>[2x]MAPLENNYNESLNKSKDAIDDKTWSKLFPSIVSDPDRSSNFMIRAIYVVFSAVLRQRNILEKEYFSKNYITE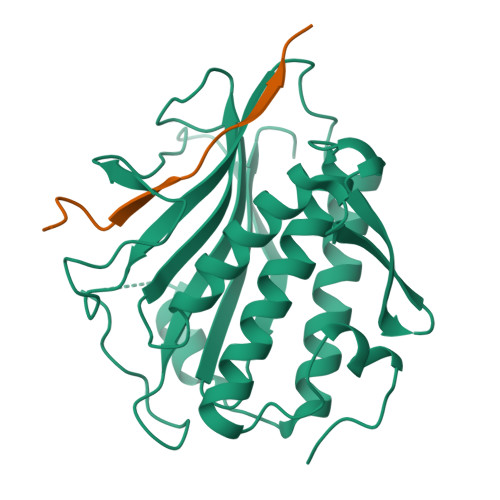NLSCMTLSFKNLRAHQIAQLLRAAGDATKDGFLKEISLVVTEHDGDVEAIEVFSMKFIYFENGGVVARLSTDNNDQEDPHFAELAQLRYEGAESVRDQMVTIVRSVQFLCTKVLEPLPAEFTANFRLKYTNDAPSNFRIDGFDDSSTFYTLPDGIQSVTIGHLRPGHHAAHMQCWSKSMSD;>[2x]SNARDSPYGLSQGITKKNKD> GSHMEAWFNEKSKELTTEIDNNIEQISSYKSEITEL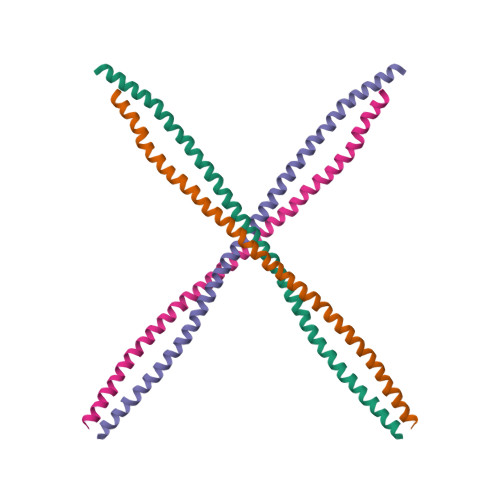RRNVQALEIELQSQLALKQSLEASLAETEGRYCVQLSQIQAQISALEEQLQQIRAETECQNTEYQQLLDIKIRLENEIQTYRSLLEGE;> ESLYQSKYEELQITAGRHGDSVRNSKIEISELNRVIQRLRSEIDNVKKQISNLQQSISDAEQRGENALKDAKNKLNDLEDALQQAKEDLARLLRDYQELMNTKLALDLEIATYRTLLEGE> MGSSHHHHHHSSGENLYFQGSHMTATATSAKAAAPACPRFDDPVHAAADPRVDVERITPDPVWRTTCGTLYRSDSRGPAVVFEQGFLPKDVIDGQYDIESYVLVNQPSPYVSTTYDHDLYKTWYKSGYNYYIDAPGGVDVNKTIGDRHKWADQVEVAFPGGIRTEFVIGV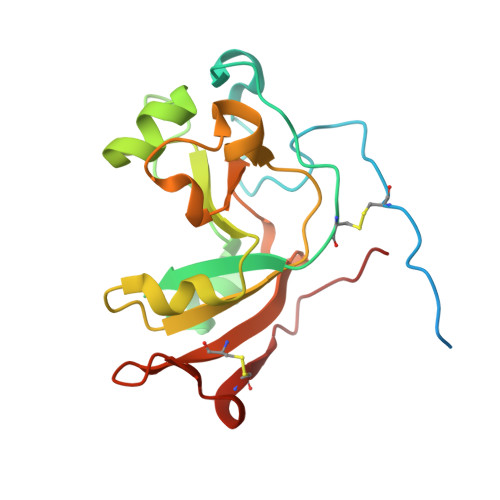CPVDKKTRTEKMSECVGNPHYEPWH>MSNQELLQLAVNAVDDKKAEQVVALNMKGISLIADFFLICHGNSEKQVQAIAHELKKVAQEQGIEIKRLEGYEQARWVLIDLGDVVVHVFHKDERAYYNL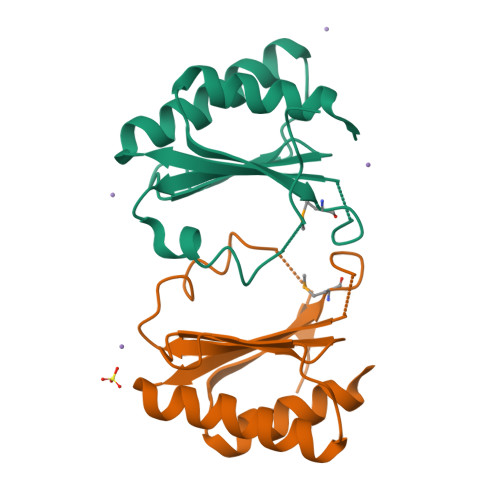EKLWGDAPTVELEGVISLEHHHHHH[2x]>MGHHHHHHHHEFIPSNTDYPGPHHFEVTFQQSSTAKFATWTYSPLLKKLYCQIAKTCPIQIKVSTPPPPGTAIRAMPVYKKAEHVTDVVKRCPNHELGRDFNEGQSAPASHLIRVEGNNLSQYVDDPVTGRQSVVVPYEPPQVGTEFTTILYNFMCNSSCVGGMNRRPILIIITLEMRDGQVLGRRSFEGRICACPGRDRKADEDHYREQ[2x]

The p53 family of transcription factors is composed of the proteins p53, p63 and p73 (1–3) that share an N-terminal transactivation domain (TA), a central sequence-specific DNA-binding domain (DBD) and an oligomerization domain (OD) within the C-terminal domain. The p53-family response element (RE) has a loose consensus which, based largely on in vitro binding studies, consists of two decameric ½-sites separated by a short spacer (n): RRRCWWGYYY-(n)-RRRCWWGYYY (R = purine; W = A/T; Y = pyrimidine; n = 0–13, although for the majority of validated REs have n < 3). Similar to p53, human p73 DBD was shown to self-assemble as a tetramer (dimer of dimers) on a full-site RE. The crystal structures of all the members of the p53 family show that the DNA-recognition residues are conserved across the family.

The crystal structure of the p73 S139F DBD in complex with the GAACA full-site RE also shows that loop L1, where K138 and the mutation S139F are located, is important for RE recognition. The configuration of the protein–DNA tetramer complex is consistent with the C2 molecular symmetry found in the structures of the WT DBDs of the three members of the p53 family. As mentioned, the overall structure of the WT and S139F mutant is alike with a root mean square deviation (r.m.s. dev.) between the α carbons of the WT p73 DBD and the S139F mutant of only 1.15. Loop L1 carries the mutation S139F that is in close proximity to the first purine nucleotide of the ½-site RE. However, loop L1 in the S139F mutant is moved further away from the base pairs in comparison with loop L1 in WT p73 DBD. In both monomers A (D) and B (C), the Phe139 residue in the p73 DBD S139F mutant is rotated away from the DNA molecule owing to the hydrophobic repulsion between the charged phosphate in the DNA backbone and the aromatic phenylalanine ring. The S139F mutation changes the conformation of loop L1 by removing the hydrogen-bonds from K138 and S139 that contact DNA in the WT protein. As a result of loop S7-S8 movement towards the adjacent monomer, the total buried tetramerization interface increases from 979 Å2 in the WT tetramer to 1188 Å2 for the mutant S139F tetramer. Our main structural observation is that the mutation S139F increases the flexibility of loop L1, together with more subtle structural rearrangements in the N-terminus and the loops S3-S4 and S7-S8. The observation that p73 S139F DBD has a much higher Kd than the WT p73 for the GAACA ½-site RE correlates with the destabilization of loop L1 in the crystal structure of the mutant with the GAACA RE.> HMLSDEQMQIINSLVEAHHKTYDDSYSDFVRFRPPVREGPVTRSASRAASLHSLSDASSDSFNHSPESVDTKLNFSNLLMMYQDSGSPDSSEEDQQSRLSMLPHLADLVSYSIQKVIGFAKMIPGFRDLTAEDQIALLKSSAIEIIMLRSNQSFSLEDMSWSCGGPDFKYCINDVTKAGHTLELLEPLVKFQVGLKKLKLHEEEHVLLMAICLLSPDRPGVQDHVRIEALQDRLCDVLQAYIRIQHPGGRLLYAKMIQKLADLRSLNEEHSKQYRSLSFQPEHSM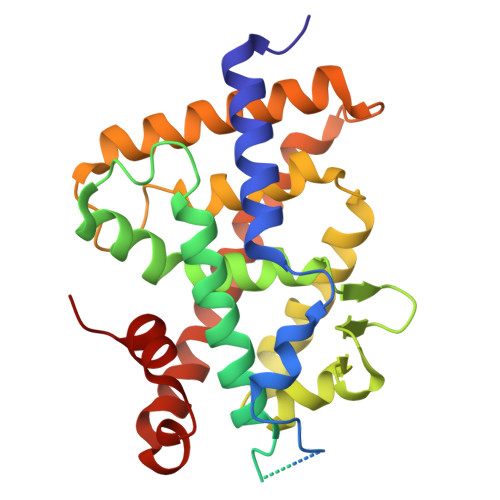QLTPLVLEVFGSEVS> GMSIYNSIGKQYSQTRVPDIRIVNAIINLLNLPKGSVIADIGAGTGGYSVALANQGLFVYAVEPSIVMRQQAVVHPQVEWFTGYAENLALPDKSVDGVISILAIHHFSHLEKSFQEMQRIIRDGTIVLLTFDIRLAQRIWLYDYFPFLWEDALRFLPLDEQINLLQENTKRRVEAIPFLLPHDLSDLFAAAAWRRPELYLKAEVRAGISSFALANQDLVEKGLELLTADLNNGEWIRKYGEIHHLQEIDIGYRFIY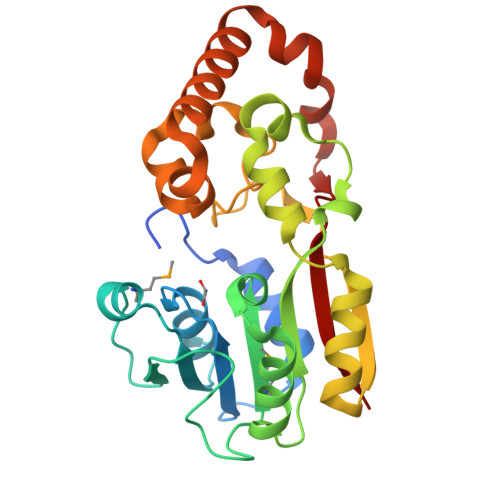TTLDK>[2x]KENKKLLCRKCKALACYTADVRVIEESHYTVLGDAF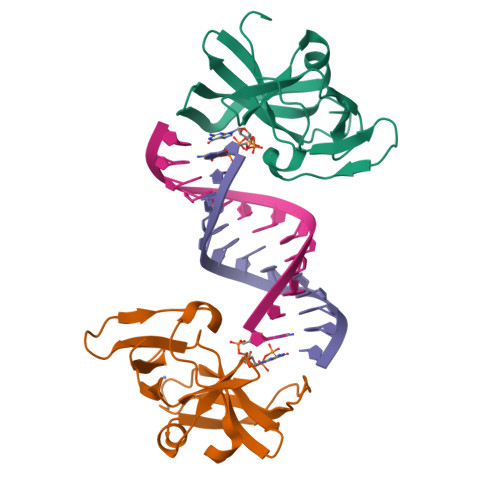KECFVSRPHPKPKQFSSFEKRAKIFCARQNCSHDWGIHVKYKTFEIPVIKIESFVVEDIATGVQTLYSKWKDFHFEKIPFDPAEM>[2x]GAMGGMHLVGVLDIAKDILKANKRLADKNRKLLNKHGVVAFDFMGAIGSGKTLLIEKLIDNLKDKYKIACIAGDVIAKFDAERMEKHGAKVVPLNTGKECHLDAHLVGH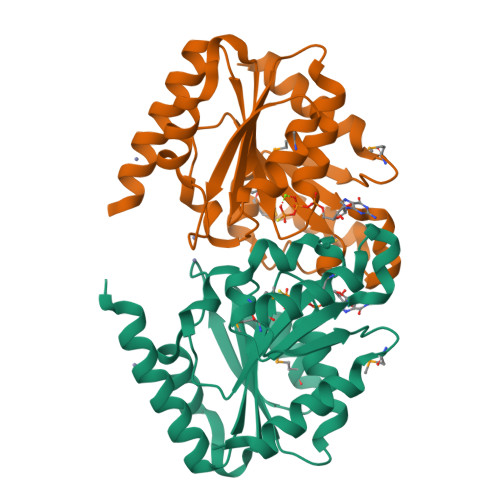ALEDLNLDEIDLLFIENVGNLICPADFDLGTHKRIVVISTTEGDDTIEKHPGIMKTADLIVINKIDLADAVGADIKKMENDAKRINPDAEVVLLSLKTMEGFDKVLEFIEKSVKEVK> ANIVGGIEYSINNASLCSVGFSVTRGATKGFVTAGHCGTVNATARIGGAVVGTFAARVFPGNDRAWVSLTSAQTLLPRVANGSSFVTVRGSTEAAVGAAVCRSGRTTGYQCGTITAKNVTANYAEGAVRGLTQGNACAGRGDSGGSWITSAGQAQ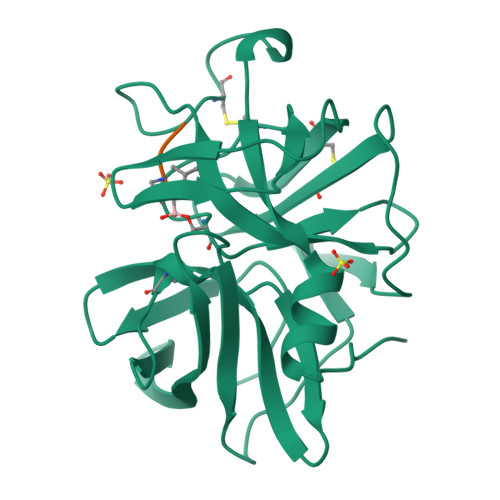GVMSGANVQSNGNNCGIPASQRSSLFERLQPILSQYGLSLVTG;> XAAPL>UGCGUCGCUCCGGAAAAGUCG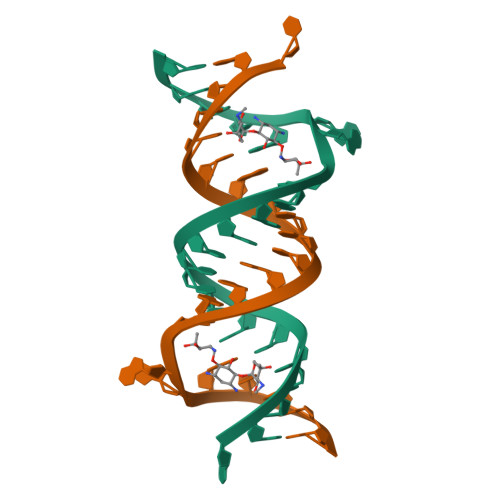C[4x]>MHHHHHHSSGSSSTGSSAAAVASKQRRRSSYAFNNGNGATNLNKSGGKKF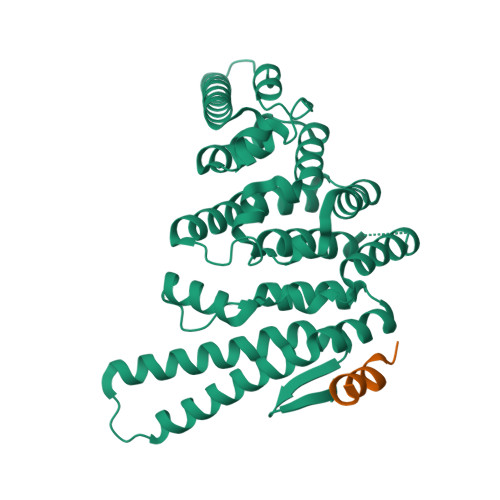ILELIETVYEEILDLEANLRNGQQTDSTAMWEALHIDDSSYDVNPFISMLSFDKGIKIMPRIFNFLDKQQKLKILQKIFNELSHLQIIILSSYKTTPKPTLTQLKKVDLFQMIILKIIVSFLSNNSNFIEIMGLLLQLIRNNNVSFLTTSKIGLNLITILISRAALIKQDSSRSNILSSPEISTWNEIYDKLFTSLESKIQLIFPPREYNDHIMRLQNDKFMDEAYIWAFLASLAASGKLNHQRIIIDEVRDEIFATINEAETLQKKEKELSVLPQRSQELDTELKSIIYNKEKLYQDLNLFLNVMGLVYRDGEISELK[2x];>SSSPGQLLDILNSK[2x]(2R)-3-[(2-chlorophenyl)amino]-2-cyano-3-thioxo-N-[3-(trifluoromethyl)phenyl]propanamide | C17 H11 Cl F3 N3 O S | 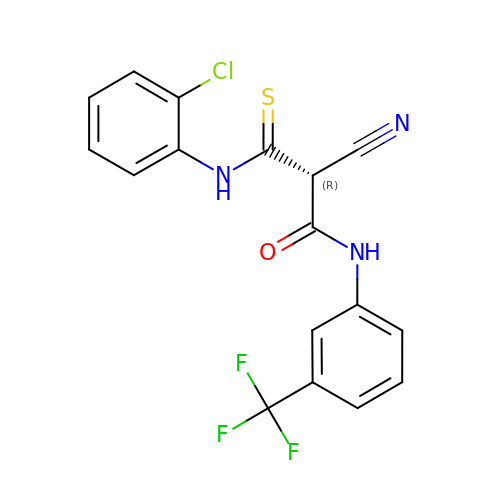JBTPUMQIJZGWRT-GFCCVEGCSA-N> VYFLKKKKNKILTIALVASLAASVSFGSVLYYSFSDNHISFDTSSNGITDAELAPINNAINDAIVSNRDNKLKPSEEKIIKETEKKIEEKIIIPPAKKEEKIEAAKPIPKPVVRKPETKITSPKITRRKQTITIAGIEVEAEIEGPPGFVTHQRDKDRKISNPTKPYQNHTVNKILSVKVTDKLKEQVAKDALSGGNGYDEGVGLFNNSIFNVFKEEFNSGKELNDILSSLESVARQNSGAFQNTLERYKKMLDSNNVINFLKSEAQKEYPKLKSKFQTKNQEYIWLIANLDQSKFTKIASTSEKYLEKGLTISPRSAFINEAGEIDSNGWGPPDEYNTVTSRLRRDNSEYRVFDYDEYYSRSSDRIANGTYPGWVKEDVSEPYSKKYNFKASDGIRFSKLERINPNPAKGKLNSGLVLDLDVSNDEAYRRSKELIEKLQKDGEQITSYRIKNMGEKNSDQAFKDILGALPKDIQQLELFFSDKATNTASLIALENKNIKELSLYTSGNSLKKAWSYNPLALRNTTWINTIDYNVSAEYSSHDKITTRITFNTLAFDQEDFSNGSYERINDGLRMVYYARNNEPFFQGGHGPGLEPDKKLGQNSYPTGLDFSRVTGIKSLKGLRFDDDLDTSNEPRKITELTLYNNESYFEISSDELNEANLQHLSTGEGNPEKPKIHFSNGNNTTSIRISGKTLLSDEGRRNLDKYFEYNESLRNSGKQIQIPNGSDELKKQLEGWGYKVSTASDRSFT;> MKRLNKLLMYISSSTLLLPITLLVACTPSKVVAKPINDDEFNKLIDSIKTENDLLKYADIRFKNPNGADTKKEDIIPSQLKSENISITFKGKYQGQISAVVTNVDVDRTNPFAVQNEATIFVQFKNLKTNTSKPISITIKGLNQKGNFDASGNIVVDDFAYFGGTSGYDEYTKKDQKSRFDYDNERYMTRLKSQFGNSSNSINLKEYRGLETKQENIKKFDDQAAISNFDTYYNAALKGFTLPVYGSDGKVSGLKIYEGAEIGKGPSVVDSLGRNEKAKTVGLARTLPNEEYKTSAIQTFQTNFTIYKDYEKEIEEAEDNIKLFDSWNEQQIQSYISAQLTQLRLNYEDEVSQIDREISQTQPDKTTILSNLNQKKSKIESEYQKELSTISKLNKDSLKEWQRKEIEKYNEKKKEKTFQISESGTMWIMDYLDENAGKNPTKFYFGTNSHVAKGIKDGMVSFSLTRLNSEVKVGQTFKLNGHDSNFTKFTFSPINGNKLEDAVTAIFHATDFINENSSPLKLLDSEQKSKYNGAGIFADFAIVEVDFAKLLDKGKYSYSVWSASNDITNQYETEQNKLISKITNNYSESDKKVKFFSDSLLNEQTYAKFDRPLDFDPKKEDELKKYNDLDSLYIVGYPTAYKDFYLDQYEDEKQLKNKKYDFSLWINSEYKFYNKLINKEGSTNSFKEYETGKGNFFSYQIGYRS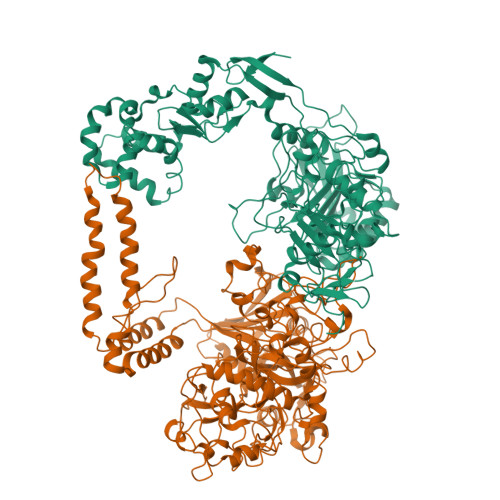FIDKPGLTDAFITVNKVGKKLYSLKDKNKNEVKKYFNYGLEILPRFYAPAGGASGSSVRTKDNKLLAVYHASNETARTGLAVAFRSDGYDYKNLFGDYKLGQYDLIYGGGKDQQKEKSYREVMNKMYSGKKSALFQNGFTDDKIPSEFKFNNGTQN>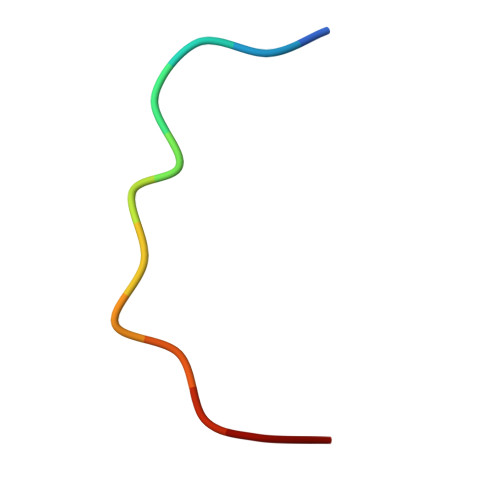 GTGGSTGTTSAG> VRKCLSDTDCTNGEKCVQKNKICSTIVEIQRCEKEHFTIPCKSNNDCQ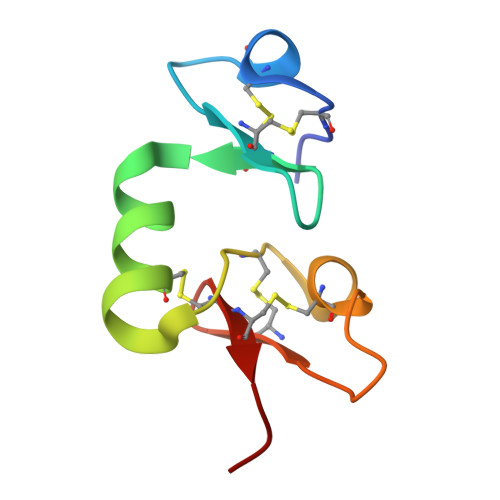VWAHEKICNKGCCWDLL>NAQFLHTQVGRGLLGAVVNPLGEVTDKFAVTDNSEILYRPVDNAPPLYSERAAIEKPFLTGIKVIDSLLTCGEGQRMGIFASAGCGKTFLMNMLIEHSGADIYVIGLIGERGREVTETVDYLKNSEKKSRCVLVYATSDYSSVDRCNAAYIATAIAEFFRTEGHKVALFIDSLTRYARALRDVALAAGESPARRGYPVSVFDSLPRLLARPGKLKAGGSITAFYTVLLEDDDFADPLAEEVRSILDGHIYLSRNLAQKGQFPAIDSLKSISRVFTQVVDEK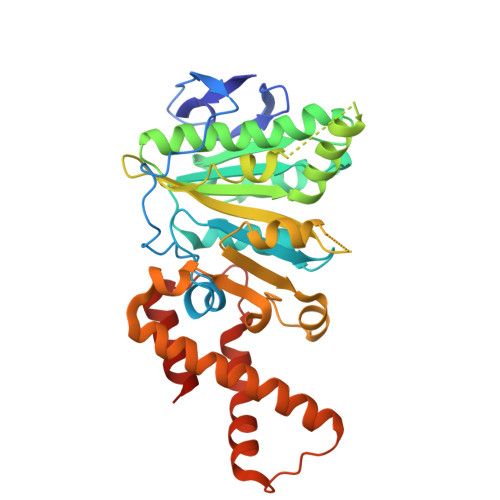HRIMAAAFRELLSEIEELRTIIDFGEYKPGENASQDKIYNKISVVESFLKQDYRLGFTYEQTMELIGETIR[2x]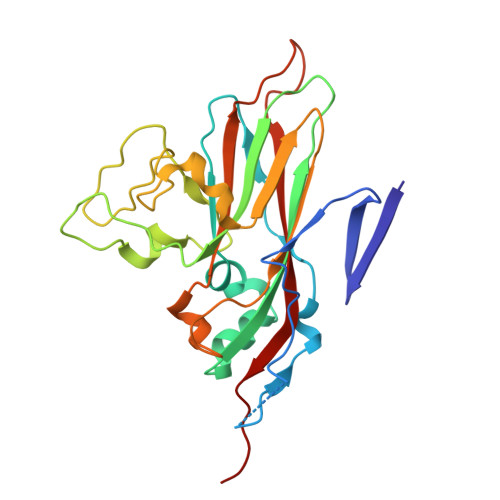> RVRSITLGNSTITTQECANVVVGYGVWPTYLNDDEATAEDQPTQPDVATCRFYTLESVMWQQSSPGWWWKFPDALSNMGLFGQNMQYHYLGRAGYTVHVQCNASKFHQGCLLVVCVPEAEMGCATLANKPDQKSLSNGETANMFESQNSTGQTAVQANVINAGMGVGVGNLTIFPHQWINLRTNNSATIVMPYINSVPMDNMFRHNNFTLMIIPFAPLSYSTGATTYVPITVTVAPMCAEYNGLRLA>[2x]GSMSLPPIRLPSPYGSDRLVQLAARLRPALCDTLITVGSQ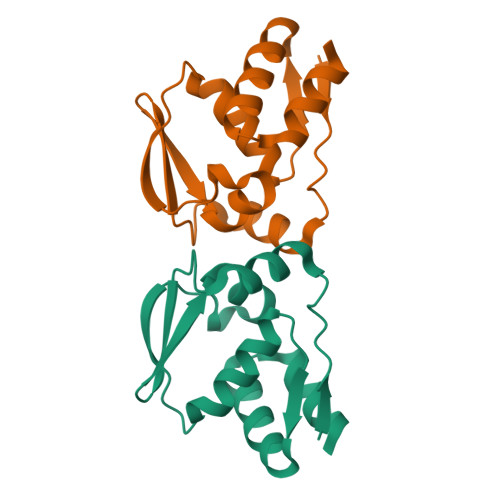EFPAHSLVLAGVSQQLGRRGQWALGEGISPSTFAQLLNFVYGESVELQPGELRPLQEAARALGVQSLEEACWRARGDRA3-[(2-methylphenyl)methylamino]pyrazine-2-carboxamide 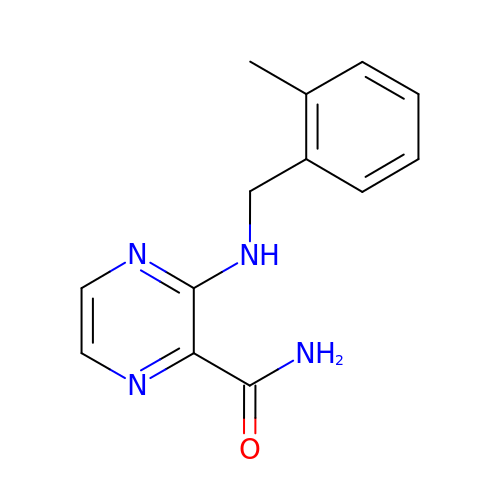| C13 H14 N4 O | RDJWFRDXOMNSOD-UHFFFAOYSA-N> GACLSIPNFPVHITGKTQQLHVGPKPSIARFSFNPFDLGTVFNRFQSLCAHLEGYSGDLIVNWLVTCSALTNARLYIIPVYDNYSFEKFSEEKLIQCKYEFKQISLVRKGTVHIPFVNWFGSYSRTRFPKLLFYFPNGVSGPSGEKIHVTVQLDRI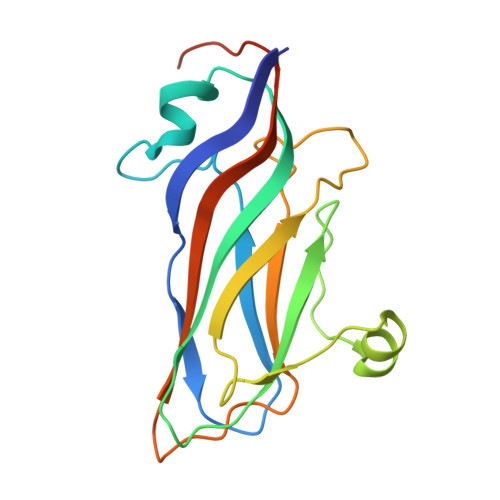LNFSGLGHRLFKEIGPLVGE(2R,4R)-N~1~-(4-CHLOROPHENYL)-N~2~-[2-FLUORO-4-(2-OXOPYRIDIN-1(2H)-YL)PHENYL]-4-METHOXYPYRROLIDINE-1,2-DICARBOXAMIDE | C24 H22 Cl F N4 O4 | 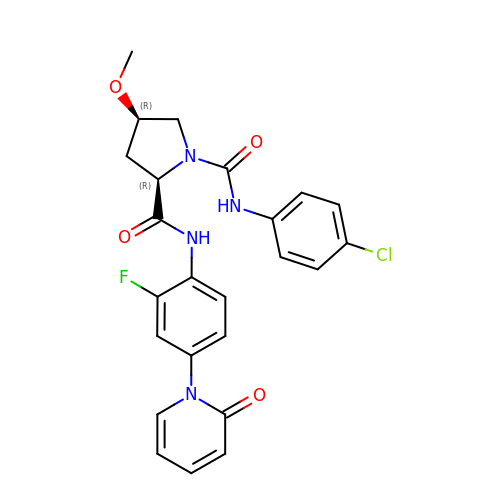QQBKAVAGLMGMHI-WIYYLYMNSA-N> GHMDYLFKLLLIGDSGVGKTCVLFRFSEDAFNSTFISTIGIDFKIRTIELDGKRIKLQIWDTAG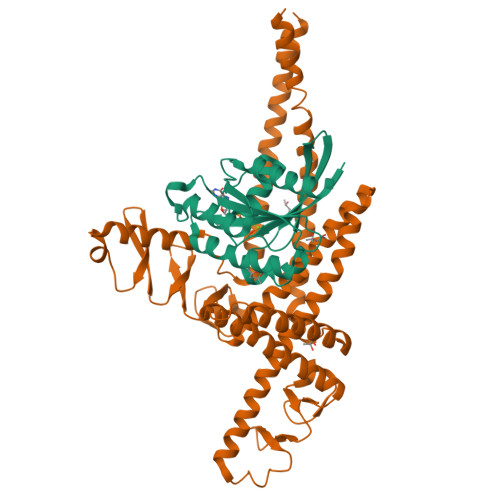QERFRTITTAYYRGAMGIMLVYDITNEKSFDNIRNWIRNIEEHASADVEKMILGNKCDVNDKRQVSKERGEKLALDYGIKFMETSAKANINVENAFFTLARDIKAKMDKK;> GMLDEYEQAIKRAQENIKKGEELEKKLDKLERQGKDLEDKYKTYEENLEGFEKLLTDSEELSLSEINEKMEAFSKDSEKLTQLMEKHKGDEKTVQSLQREHHDIKAKLANLQVLHDAHTGKKSYVNEKGNPVSSLKDAHLAINKDQEVVEHEGQFYLLQKGQWDAIKNNPAALEKAQKDYSQSKHDLATIKMEALIHKLSLEMEKQLETINNLIMSTDPKENEEATKLLHKHNGLNLKLANLQDMLAVHRKEKSFFNEKGEEVTSLNDAHYVIGKDQQLFNLGGKFYPIHKEQKILEKDGKFYLLKQGEDWESIKDSPEKQKKAEHDFHKLQYETPMTVKKLVHHNKGLETTIHKERVEETKQQLEDNGKEKIEIANNISKLQS> MISGWGARPEEQYEMIRAAVPPSEAEPRLQ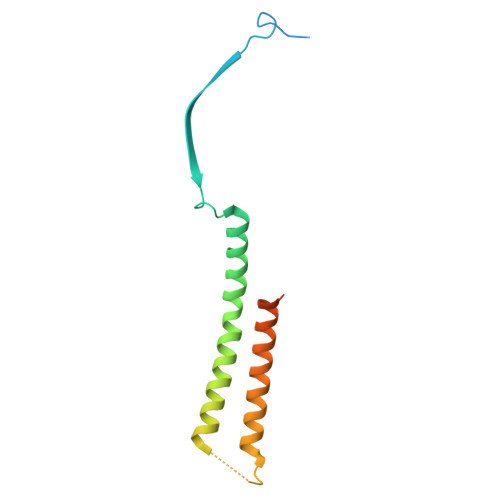EALVVVNALLPAPITLDDALGSLDDTRRLVKARALARTYHACMVNLERLARHHPGLEAPTIDGAVAAHQDKMRRLADTCMATILQMYMSVGAADKSADVLVSQAIR> ETGQCKILRCNAEYVSSTL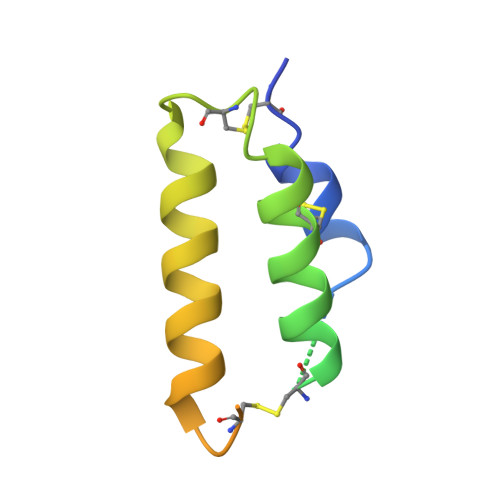SLRGGGSSGALRGGGGGGRGGGVGSGGLCRALRSYALCTRRTARTCRGDLAFHSAVHGIEDLMIQHNCSRQGPTAPPPPRGPALPGAGSGLPAPGTKHHHHHH>[2x]MDIVAPDRTRIAPEIDRDEALEGDRESDPALASTREWQLEDMPRWQDELTVRGLVAALLIGFIYTVIVMKIALTTGLVPTLNVSAALLSFLALRGWTRLLERFGVVSRPFTRQENTIVQTCGVACYTIAFAGGFGSTLLGLNKKTYELAGDSPGNVPGSWKEPGIGWMTGFLLACSFGGLLTLIPLRQVLVVDYKLVYPSGTATAILINGFHTDQGDKNSRKQIRGFLKYFGGSFLWSFFQWFYTGGDACGFVQFPTFGLKAWKQTFYFDFSMTYVGAGMICPHIVNISTLLGAIISWGIMWPLISKNKGDWYPAKVPESSMKSLYGYKAFICIALIMGDGMYHFIKIVGITAMSMYRQFSHKQVNNKAKNADDTVSL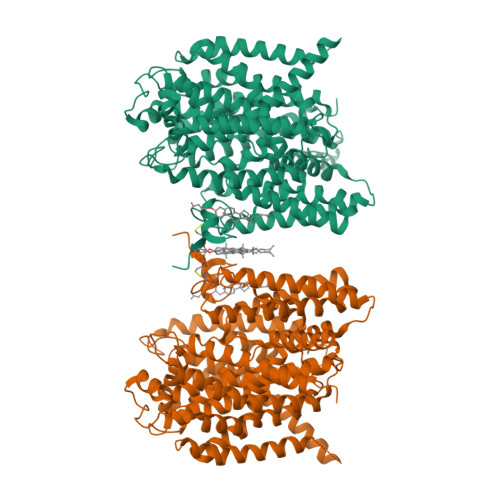EELHRQEIFKRGHIPSWMAYAGYALFSVLAVVTIPVMFKQVKWYYVVIAYVVAPMLGFANSYGTGLTDINMGYNYGKIALFVFAGWAGKENGVIAGLVAGTLVKQLVLISADLMQDFKTSYLTQTSPKSMMIAQVVGTAMGCIVSPLTFMLFYKAFDIGNPDGTWKAPYALIYRNMAILGVEGFSVLPKYCIVISGGFFAFAAILSITRDVMPHKYAKYVPLPMAMAVPFLVGGSFAIDMCLGSLIVFAWTKINKKEAGFMVPAVASALICGDGIWTFPASILALAKIKPPICMKFLPAATSAAHHHHHHHH In this work, we exhaustively probe the ability of all 36 immobile HJ sequences to form DNA crystals in two different designed systems. Three separate self-assembling DNA crystal systems are described in this report: the “4 × 5” and “4 × 6” designs (collectively referred to as the 4 × N systems), and a third construct with a “scrambled” sequence variant of the 4 × 6 lattices. Self-assembly was mediated by three constituent oligonucleotides: (S1) containing four sequence repeats of either 5 or 6 bases; (S2) composed of 21 bases containing complementary regions to both (S1); and (S3) which forms the second junction crossover. The HJ serves as the fundamental component at the core of each unit, and the ultimate assembly of the full lattice is facilitated by the complementary 2-base sticky ends that tail each duplex.

To investigate this possibility, we designed “scrambled” sequences with targeted base substitutions, while maintaining GC content, along each “stem”. Contrary to the buffer preference observed with the native P32 crystals, the scrambled systems exhibited an exclusive preference towards low salt buffers, much like the native R3 crystals. Remarkably, only J1 and J2 retained the P32 symmetry, with all others yielding an R3 lattice. There appeared to be only a marginal difference in the average cell lengths in the R3 scramble crystals (a = b = 113.04 c = 51.10) relative to the native 4 × 6 sequences: the a, b axis trended ~2 Å shorter and c ~1.3 Å longer, whereas in the J1 and J2 cases, the crystals were in good agreement with the original 4 × 6 motif. The most significant difference between the individual junctions observed in MD simulations was their ability to form distinct potassium ion binding sites near the junction branching point.

> CCGTCT;> GAACGACACAGACGGTGACTC;> TCGAGTCA;> GTGTCGT>[8x]SKGLEDSSTISFITWNIDGLDGCNLPERARGVCSCLALYSPDVVFLQEVIPPYCAYLKKRA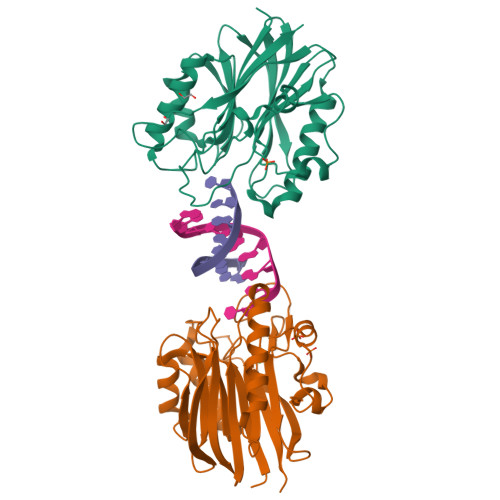ASYTIITGNEEGYFTAILLKKGRVKFKSQEIIPFPNTKMMRNLLCVNVSLGGNEFCLMTSHLESTREHSAERIRQLKTVLGKMQEAPDSTTVIFAGDTNLRDQEVIKCGGLPDNVFDAWEFLGKPKHCQYTWDTKANNNLRIPAAYKHRFDRIFFRAEEGHLIPQSLDLVGLEKLDCGRFPSDHWGLLCTLNVVL;> SNVKTENNDHINLKVAGQDGSVVQFKIKRHTPLSKLMKAYCERQGLSMRQIRFRFDGQPINETDTPAQLEMEDEDTIDVFQ>GAIIGL[2x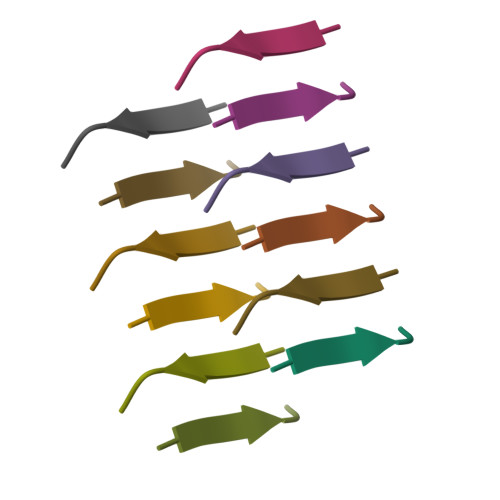]> STIHNEAELGD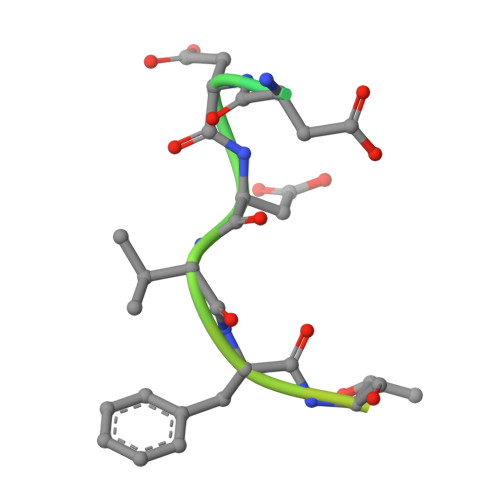DDVFTTATDSSSNSSQKRE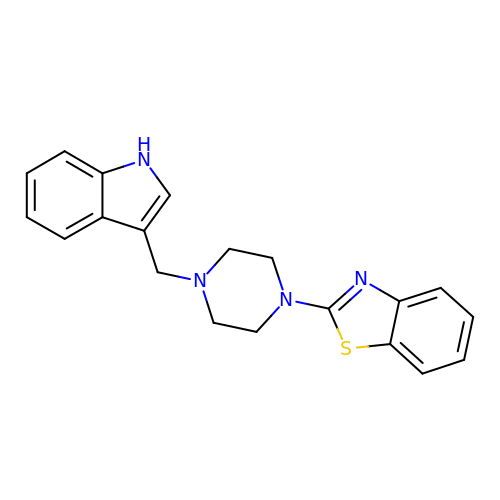2-[4-(1~{H}-indol-3-ylmethyl)piperazin-1-yl]-1,3-benzothiazole | C20 H20 N4 S | RCRIPVWIXYCQFS-UHFFFAOYSA-N>[4x]MKAQELGIKIGVFKPGKRNKITDVKGVKVGHVTLIKGKGKLIPGKGPVRTGVTAILPHEGNIYKEKVLAGAFVMNGYSKPVGLIQLWELGTIETPIILTNTLSIGTAVEGLLDYILEENEDIGVTTGSVNPLVLECNDSYLNDIRGRHVKREHVVEAIKRADEDFEEGAVGAGTGMSAFEFKGGIGSASRIVEIEGKKYTVGALVLSNFGRREDLTIA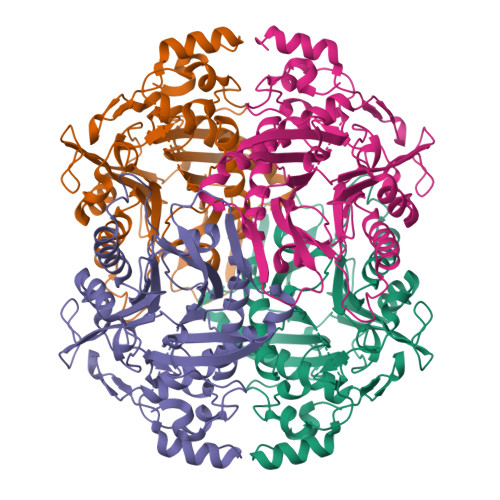GVPVGLELKNWPGRGGEGKGSIIMIIATDAPLTGRQLNRVAKRAIVGLARTGGYAYNGSGDIAVAFSTANRIKHYEKEVIEIKALPDSVISPLFKATAEAVEEAIINSLLEARTMDGRDNHVRYALPKEELLRIMRRYGRLEE>[4x]SKMSDVKCTSVVLLSVLQQLRVESSS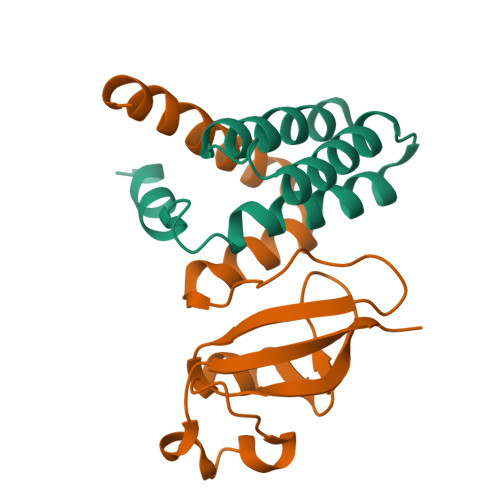KLWAQCVQLHNDILLAKDTTEAFEKMVSLLSVLLSMQGAVDINKLCEEMLDNRATLQ;>EDKRAKVTSAMQTMLFTMLRKLDNDALNNIINNARDGCVPLNIIPLTTAAKLMVVIPDYNTYKNTCDGTTFTYASALWEIQQVVDADSKIVQLSEISMDNSPNLAWPLIVTALRANSAVKLQ[4x]> MSQKNGIATLLQAEKEAHEIVSKARKYRQDKLKQAKTDAAKEIDSYKIQKDKELKEFEQKNAGGVGEL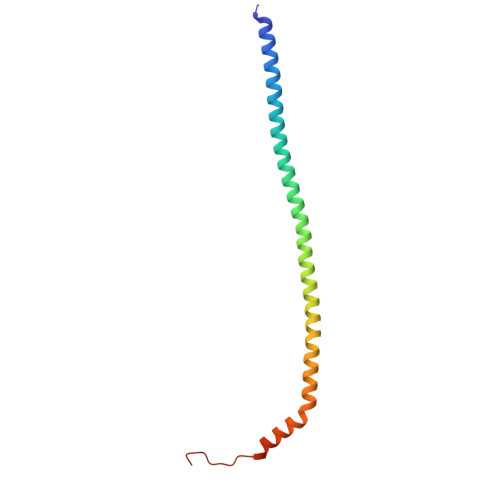EKKAEAGVQGELAEIKKIAEKKKDDVVKILIETVIKPSAEVHINAL>[2x]GPLGSPEFQRTKPFSVPNIPMNLMSNSRVPMLIDGMMVSNDQNQVPQ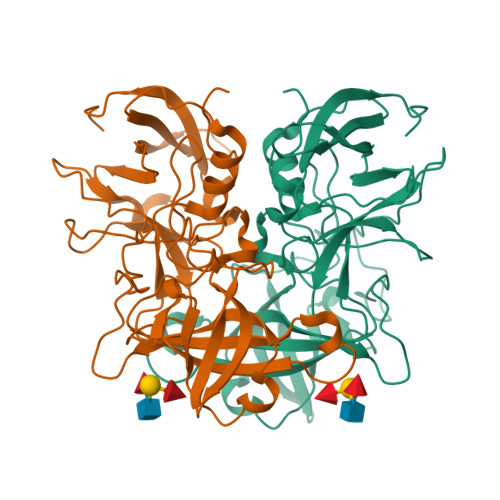FQNGRVTLDGQLQGTTTVSAACIARMRGRIFNNNGNYGVNLAELDGNPYHAFDSPAPLGFPDFGNCDLHMTFVKINPTELSTGDPSGKVVIHSYDATFAPHLGTVKLEDNNELDQFVGKEVVLELTWVSNRTGATLNLWAVPNYGSNLTQASQLAPPIYPPGFGEAIVYFTSTFPTVSNPKVPCTLPQEFVSHFVNEQAPTRGDAALLHYVDPDTHRNLGEFKMYPEGYMTCVPNAGGGPQTLPINGVFVFISWVSRYYQL>[4x]MKIAVIGQSLFGQEVYCQLRKEGHEVVGVFTIPDKDGKADPLGLEAEKDGVPVFKFPRWRARGQALPEVVAKYQALGAELNVLPFCSQFIPMEVINAPRHGSIIYHPSLLPRHRGASAINWTLIHGDKKGGFTIFWADDGLDTGDLLLQKECEVLPDDTVSTLYNRFLFPEGIKGMVQAVRLIAEGTAPRCPQSEEGATYEGIQKKETAKINWDQPAEAIHNWIRGNDKVPGAWTEACGQKLTFFNSTLNTSGLSTQGEALPIPGAHRPGVVTKAGLILFGNDDRMLLVKNIQLEDGKMMPASQFFKGSASSDLELTEAELATAEAVRSSWMRILPNVPEVEDSTDFFKSGAASVDVVRLVEEVKELCDGLELENEDVYMATTFRGFIQLLVRKLRGEDDESECVINYVEKAVNKLTLQMPYQLFIGGEFVDAEGSKTYNTINPTDGSVICQVSLAQVSDVDKAVAAAKEAFENGLWGKINARDRGRLLYRLADVMEQHQEELATIEALDAGAVYTLALKTHVGMSIQTFRYFAGWCDKIQGATIPINQARPNRNLTLTKKEPVGVCGIVIPWNYPLMMLSWKTAACLAAGNTVVIKPAQVTPLTALKFAELTLKAGIPKGVVNILPGSGSLVGQRLSDHPDVRKIGFTGSTEVGKHIMKSCALSNVKKVSLELGGKSPLIIFADCDLNKAVQMGMSSVFFNKGENCIAAGRLFVEESIHNQFVQKVVEEVEKMKIGNPLERDTNHGPQNHEAHLRKLVEYCQRGVKEGATLVCGGNQVPRPGFFFQPTVFTDVEDHMYIAKEESFGPIMIISRFADGDVDAVLSRANATEFGLASGVFTRDINKALYVSDKLQAGTVFINTYNKTDVAAPFGGFKQSGFGKDLGEAALNEYLRIKTVTFEY

Putative tumor suppressor ALDH1L1, the product of natural fusion of three unrelated genes, regulates folate metabolism by catalyzing NADP+-dependent conversion of 10-formyltetrahydrofolate to tetrahydrofolate and CO2. The protein exists as a homotetramer, with each 902 amino acid-long protomer organized in three distinct functional domains. Overall, in the ALDH1L1 catalysis, the 4′-PP arm of the Int domain transfers the formyl group cleaved from 10-fTHF in the folate-binding Nt domain to the Ct domain, where it is oxidized to carbon dioxide. Remarkably, the tetrameric state of ALDH1L1 is indispensable for catalysis because the intermediate domain transfers formyl between the catalytic domains of different protomers.

Subsequently, we used cryo-EM to characterize the structure of ligand-free ALDH1L1 at high resolution. A 3.7-Å map was obtained from a dataset of 86,276 particles when D2 symmetry was imposed. The rigid Ct core and four Int domains were clearly resolved in this structure, while the highly mobile Nt domains were not visible in the symmetrical map. To determine the fraction of free (not occupying substrate entrance tunnels) Int domains, we performed local 3D classification within a mask encompassing each Int domain and calculated the total number of particles that contributed to empty versus occupied classes. This analysis produced estimated average occupancies of 76% and 83% for the Int domain in the ligand-free and NADP+-bound structures, respectively. Curiously, we found that the sulfur atom of the catalytic nucleophile Cys707 in the ALDH active center was positioned closely to the sulfur atom of the 4′-PP, and the cryo-EM density between the two atoms appeared continuous. This suggested that a disulfide bond formed between the two atoms. In an attempt to resolve the Nt domain of ALDH1L1, we performed refinement of the cryo-EM dataset of ligand-free ALDH1L1 without enforcing symmetry. The resulting 4.4-Å-resolution map was very similar to its symmetrical counterpart, except that weak density for a single Nt domain became visible. This Nt domain appeared to interact with the NADP+-binding sub-domain of one of the Ct domains. Low r.m.s.d. values between the chains of this structure (0.67–0.74 Å) indicated that this interaction did not induce large structural rearrangements in the protein core.> PPGPTLRE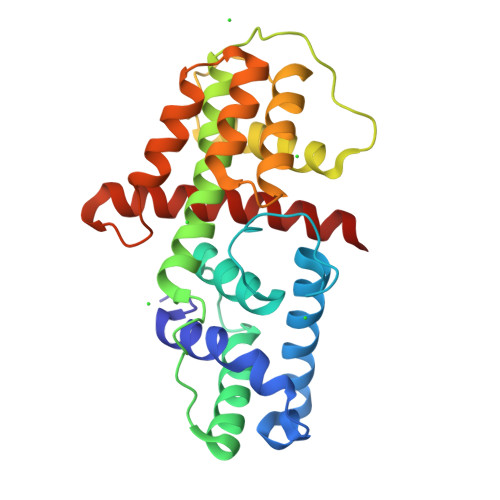LWWVFYAADRALEEPRADSGLTREEVRAVRGFREQAWKLFGSAGAPRAFIGAALGLSPLQKLAVYYYIIHRERRLSPFPALVRLVGRYTQRHGLYVPRPDDPVLADAINGLFRDALAAGTTAEQLLMFDLLPPKDVPVGSDVQADSTALLRFIESQRLAVPGGVISPEHVAYLGAFLSVLYAGRGRMSAATHTARLTGVTSLVLAVGDVDRLSAFDRGAAGAASRTRAAGYLDVLLTVRLARSQ> MIKVVVRKRPLSELEKKKKDSDIITVKNNCTLYIDEPRYKVDMTKYIERHEFIVDKVFDDTVDNFTVYENTIKPLIIDLYENGCVCSCFAYGQTGSGKTYTMLGSQPYGQSDTPGIFQYAAGDIFTFLNIYDKDNTKGIFISFYEIYCGKLYDLLQKRKMVAALENGKKEVVVKDLKILRVLTKEELILKMIDGVLLRKIGVNSQNDESSRSHAILNIDLKDINKNTSLGKIAFIDLAGSE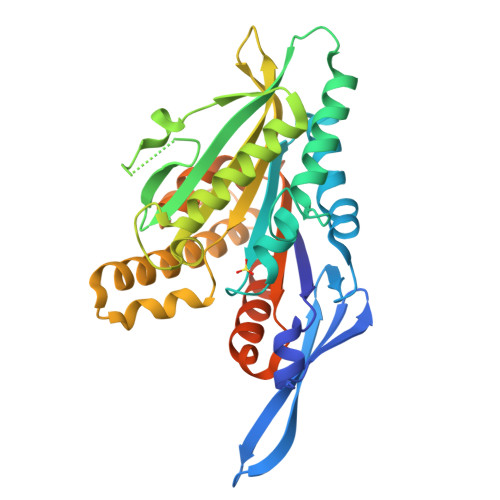RGADTVSQNKQTQTDGANINRSLLALKECIRAMDSDKNHIPFRDSELTKVLRDIFVGKSKSIMIANISPTISCCEQTLNTLRYSSRVKNKGNSKLEGKPIPNPLLGLDSSRTGHHHHHH> TKFIGCIDLHNGEVKQIVGGTLTSKKEDVPKTNFVSQHPSSYYAKLYKDRDVQGCHVIKLGPNNDDAAREALQESPQFLQVGGGINDTNCLEWLKWASKVIVTSWLF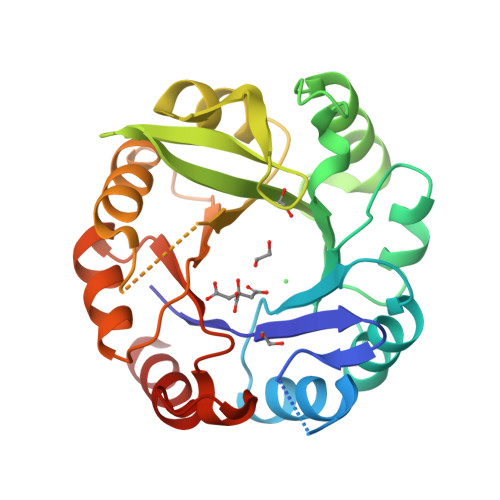TKEGHFQLKRLERLTELCGKDRIVVDLSCRKTQDGRWIVAMNKWQTLTDLELNADTFRELRKYTNEFLIHAADVEGLCGGIDELLVSKLFEWTKDYDDLKIVYAGGAKSVDDLKLVDELSHGKVDLTFGSSLDIFGGNLVKFEDCCRWNEKQG> DLGSIATWSKHAKPVACSGDWLGVRDKCFYFSDDTRNWTASKIFCSLQKAELAQIDTQEDMEFLKRYAGTDMHWIGLSRKQGDSWKWTNGTTFNGWFEIIGNGSFAFLSADGVHSSRGFIDIK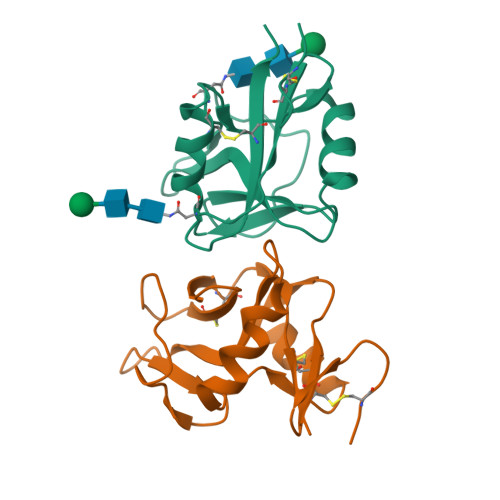WICSKPKYFLAAAHHHHHH;> DLGSSQNVNVSSLSGHNYLCPNDWLLNEGKCYWFSTSFKTWKESQRDCTQLQAHLLVIQNLDELEFIQNSLKPGHFGWIGLYVTFQGNLWMWIDEHFLVPELFSVIGPTDDRSCAVITGNWVYSEDCSSTFKGICQRDAILTHNGTSGVAAAHHHHHH>[4x]GSSPLLKSAEREKEMASMKEEFTRLKEALEKSEARRKELEEKMVSLLQEKNDLQLQVQAEQDNLADAEERCDQLIKNKIQLEA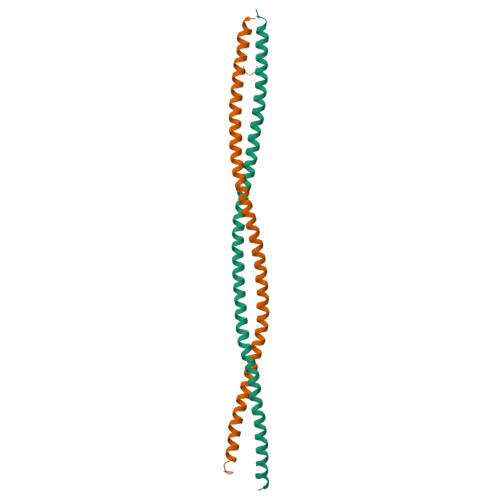KVKEMNKRLEDEEEMNAELTAKKRKLEDECSELKRDIDDLELTLAK> GHMSQWQAKQELAEAKKTATTFLNVLSKQEFDKLPSVVQEASLKKNGYDTKSVVEKYQAIYSGIQAEGVKASDVQVKKAKDNQYTFTYKLSMSTPLGEMKDLSYQSSIAKKGDTYQIAWKPSLIFPDMSGNDKISIQVDNAKRGEIVDRNGSGLAINKVFDEVGVVPGKLGSGAEKTANIKAFSDKFGVSVDEINQKLSQGWVQADSFVPITVASEPVTELPTGAATKDTESRYYPLGEAAAQLIGYTGTITAEDIEKNPELSSTGVIGKTGLERAFDKELRGQDGGSLVILDDKENVKKALQTKEKKDGQTIKLTIDSGVQQQAFAIFDKRPGSAVITDPQKGDLLATVSSPSYDPNKMANGISQKEYDAYNNNKDLPFTARFATGYAPGSTFKTITGAIGLDAGTLKPDEELEINGLKWQKDKSWGGYFATRVKEASPVNLRTALVNSDNIYFAQQTLRMGEDKFRAGLNKFIFGEELDLPIAMTPAQISNEDKFNS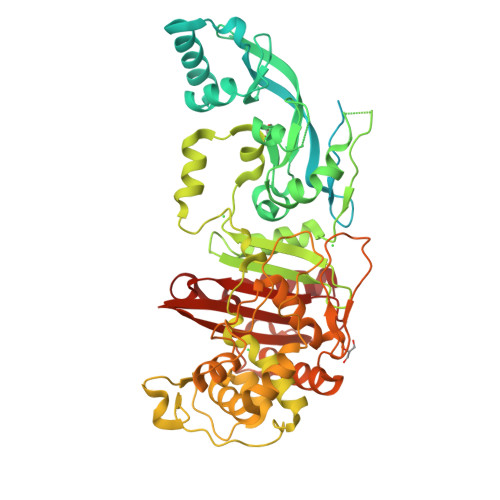EILLADTGYGQGQLLISPIQQATMYSVFQNNGTLVYPKLVLDKETKKKDNVISANAANTIATDLLGSVEDPSGYVYNMYNPNFSLAAKTGTAEIKDKQDTDGKENSFLLTLDRSNNKFLTMIMVENSGENGSATDISKPLIDYLEATIK>[6x]MGSDKIHHHHHHENLYF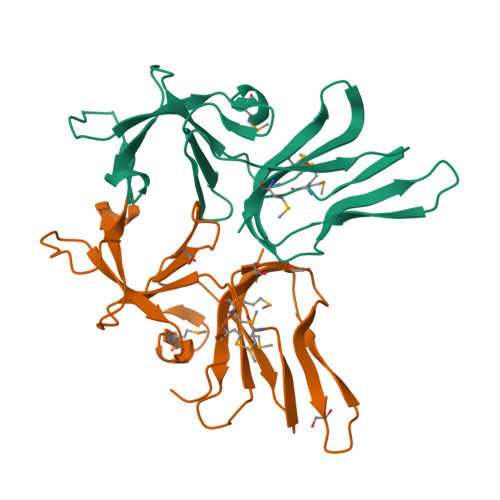QGMKIPKIYVEGELNDGDRVAIEKDGNAIIFLEKDEEYSGNGKLLYQVIYDDLAKYMSLDTLKKDVLIQYPDKHTLTYLKAGTKLISVPAEGYKVYPIMDFGFRVLKGYRLATLESKKGDLRYVNSPVSGTVIFMNEIPSERANYVFYMLEE>MNKLTIIVTYYNAEEYITGCLESIKQQRTQDFNLIIVNDGSTDQSKKLMDEAIKDYDKNIRFIDLDENSGHAHARNIALEEVETPYFMFLDADDELASYAITFYLEKFNNTDGLIAPIHSFTTQ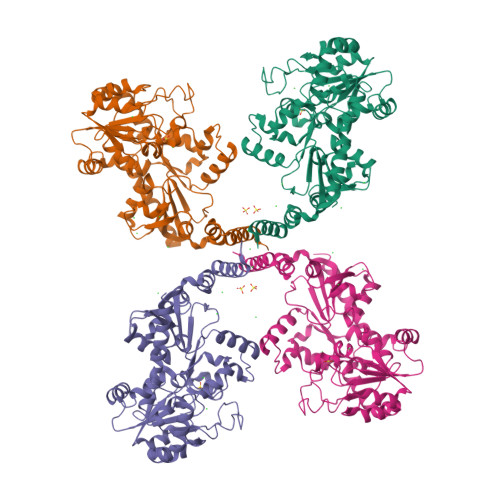RPQFVDLDRVRVEYFNAKENINSFLRKQSACNIIFRTAIVRAHHIRFNENLNTYVDWSFVLEYMKYVNKFVRIFNFPFYFRGEVYDPFETLTLSEQNFDILFKDYVNSFYDAIKRATNPKVREFIVTKMGNKIANEFEPTRYDINERYQTHKDTLVELSKFLHVHLVKNQKLINKIETILLMNNETDKAFKVNQFRKTLRHVKNIVLRRKNKERSLYDLTDKEDNVKPKTIVFESFGGKNYSDSPKYIYEYMQKYYPNYRYIWSFKNPDKNVVPGSAEKVKRNSAEYYQAYSEASHWVSNARTPLYLNKKENQTYIQTWNGTPLKRLANDMKVVRMPGTTTPKYKRNFNRETSRWDYLISPNRYSTEIFRSAFWMDEERILEIGYPRNDVLVNRANDQEYLDEIRTHLNLPSDKKVIMYAPTWRDDEFVSKGKYLFELKIDLDNLYKELGDDYVILLRMHYLISNALDLSGYENFAIDVSNYNDVSELFLISDCLITDYSSVMFDYGILKRPQFFFAYDIDKYDKGLRGFYMNYMEDLPGPIYTEPYGLAKELKNLDKVQQQYQEKIDAFYDRFCSVDNGKASQYIGDLIHKDIKEQLEHHHHHH[4x]2'-DEOXYCYTIDINE | C9 H13 N3 O4 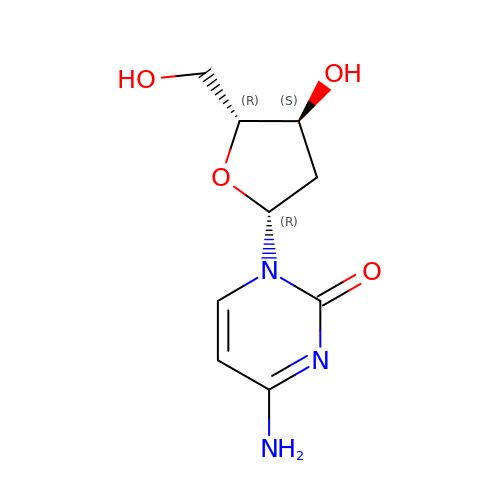| CKTSBUTUHBMZGZ-SHYZEUOFSA-N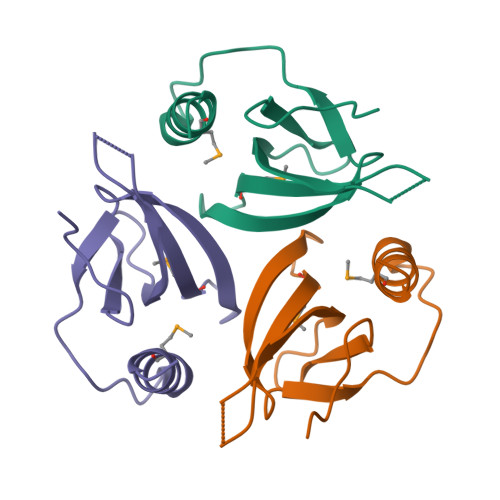> MIASKFGIGQQVRHSLLGYLGVVVDIDPVYSLSEPSPDELAVNDELRAAPWYHVVMEDDNGLPVHTYLAEAQLSSELQDEHPEQPSMDELAQTIRKQLQAPRLRN The ATP-driven mutual interplay between myosin and actin drives muscle contraction and many other forms of cellular motility, including cytokinesis and directional cargo transport; yet, our molecular understanding of how these two cytoskeletal proteins communicate with each to generate force still remains incomplete. With the aid of mutant analyses based on kinetic investigations and simulations, we identified the W-helix as an important hub coupling the structural changes of switch elements during ATP hydrolysis to temporally controlled interactions with actin that are passed to the central transducer and converter. A critical role in controlling the sequence of events associated with force production appears to be played by the W-helix, which we propose to act as kind of communication zone in the inner myosin core for coupling conformational rearrangements upon nucleotide binding to cleft closure-induced β-sheet distortions by putting a stress on β1 to β3 of the central transducer; this is important to temporally couple weak-to-strong actin-binding transitions to the initiation of the power stroke and release of hydrolysis products. To gain mechanistic insights into the proposed role of the W-helix/transducer region in mediating actin binding to product release, we followed a mutational approach and replaced the two hotspot threonines in the W-loop of the myosin-2 motor domain from D. discoideum by either two alanines (AA) or three glycines (GGG) in order to reduce the rigidity of that region during weak-to-strong transition without dramatically disturbing the fold of the protein.

Replacing the two W-loop residues by three glycines in M765GGG was expected to affect loop flexibility more drastically than with the double-alanine mutant construct M765AA. We crystallized the motor domains of the mutant myosins M765AA and M765GGG in complex with ADP∙VO32− and solved the atomic structures of the proteins to a resolution of 2.60 Å and 2.55 Å, respectively. The superimposed structures reveal that the mutants crystallized in the pre-power-stroke state adopting the same overall conformation as previously reported for the wildtype. Characteristic features of this pre-power-stroke state are the partially open actin-binding cleft, the up position of the converter, and the relay helix in a bent conformation. Only minor structural deviations from the wild-type conformation can be observed for the mutants concerning the β3, β5, and β7 strands of the central transducer, which are slightly shifted, as well as the relay helix conformation. The high resemblance of the wild-type and mutant structures, which are representative for the actin-detached conformation of myosin just prior to Pi release, and actin-rebinding suggest that the mutations have no or only a minor impact on ATP turnover if actin is absent, consistent with our hypothesis that the W-helix primarily mediates the communication between active site elements and the actin-binding region.

> MHHHHHHHDGTENPIHDRTSDYHKYLKVKQGDSDLFKLTVSDKRYIWYNPDPKERDSYECGEIVSETSDSFTFKTVDGQDRQVKKDDANQRNPIKFDGVEDMSELSYLNEPAVFHNLRVRYNQDLIYTYSGLFLVAVNPFKRIPIYTQEMVDIFKGRRRNEVAPHIFAISDVAYRSMLDDRQNQSLLITGESGAGKTENTKKVIQYLASVAGRNQANGSGVLEQQILQANPILEAFGNAKTTRNNNSSRFGKFIEIQFNSAGFISGASIQSYLLEKSRVVFQSETERNYHIFYQLLAGATAEEKKALHLAGPESFNYLNQSGCVDIKGVSDSEEFKITRQAMDIVGFSQEEQMSIFKIIAGILHLGNIKFEKGAGEGAVLKDKTALNAASTVFGVNPSVLEKALMEPRILAGRDLVAQHLNVEKSSSSRDALVKALYGRLFLWLVKKINNVLCQERKAYFIGVLDISGFEIFKVNSFEQLCINYTNEKLQQFFNHHMFKLEQEEYLKEKINWTFIDFGLDSQATIDLIDGRQPPGILALLDEQSVFPNATDNTLITKLHSHFSKKNAKYEEPRFSKTEFGVTHYAGQVMYEIQDWLEKNKDPLQQDLELCFKDSSDNVVTKLFNDPNIASRAKKGANFITVAAQYKEQLASLMATLEGGGNPHFVRCIIPNNKQLPAKLEDKVVLDQLRCNGVLEGIRITRKGFPNRIIYADFVKRYYLLAPNVPRDAEDSQKATDAVLKHLNIDPEQYRFGITKIFFRAGQLARIEEAREQRLESNEPPMDFDDDIPF>[2x]MRFWPLDATYSVVG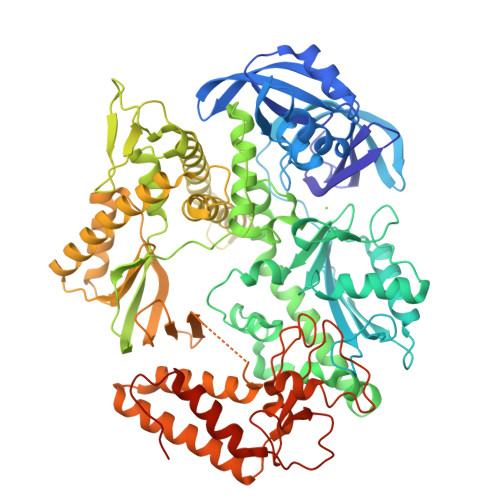GVPEVRVFGVDGEGRRVVLVDRRFRPYFYAKCDKCDASLAKSYLSRVAPVEAVEVVERRFFGRPTIFLKVVAKVPEDVRKLREAALGAPGVVDVYEADIRYYMRYMIDKGVVPCAWNVVEAREAGKLGPLPLYEVVEWAGVEEGFPPPLRVLAFDIEVYNERGSPDPLRDPVVMLAVKTSDGREEVFEAEGRDDRRVIRGFVDFVKEFDPDVIVGYNSNGFDWPYLSERAKALGVPLRVDRLGGVPQQSVYGHWSVVGRANVDLYNIVDEFPEIKVKTLDRVAEYFGVMKRSERVLIPGHKVYEYWNDPAKRPTLMRYVLDDVRSTLGLAEKLLPFLIQLSSVSGLPLDQVAAASVGNRVEWMLLRYAYRMGEVAPNREEREYEPYKGAIVLEPKPGLYSDVLVLDFSSMYPNIMMKYNLSPDTYLEPHEPDPPEGVVVAPEVGHRFRKAPTGFIPAVLKHLVELRRAVREEAKKYPPDSPEYRLLDERQRALKVMANAMYGYLGWVGARWYKKEVAESVTAFARAILLDVVEYAKRLGIEVIYGDTDSLFVKKSGAVDRLVKYVEERHGIEIKVDKDYERVLFTEAKKRYAGLLRDGRIDIVGFEVVRGDWCELAKEVQLNVVELILKSKSVGEARERVVKYVREVVERLKAYKFDLDDLIIWKTLDKELDEYKAYGPHVHAALELKRRGYKVGKGTTVGYVIVRGPGKVSERAMPYIFVDDASKVDVDYYIEKQVIPAALRIAEVLGVKESDLKTGRVEKSLLDFLG N-[2-(2-methoxy-1H-dipyrido[2,3-a:3',2'-e]pyrrolizin-11-yl)ethyl]furan-2-carboxamide | C21 H18 N4 O3 | 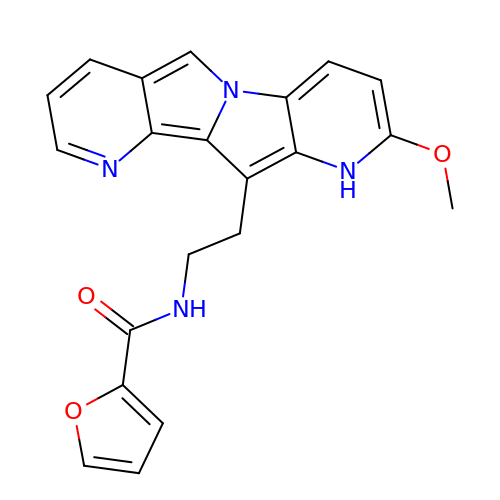WIMLBKFZRMRSHL-UHFFFAOYSA-N>MSPILAKNIVYVAQIKGQITSYTYDQFDRYITIAEQDNAEAIIIELDTPGGRADAMMNIVQRIQQSKIPVIIYVYPPGASAASAGTYIALGSHLIAMAPGTSIGACRPILGYSQNGSIIEAPPKITN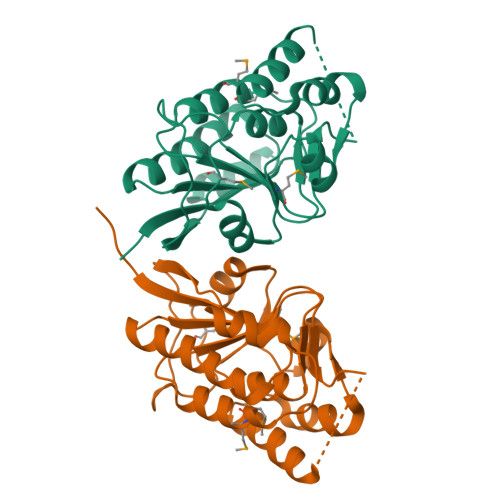YFIAYIKSLAQESGRNATIAEEFITKDLSLTPEEALKYGVIEVVARDINELLKKSNGMKTKIPVNGRYVTLNFTNVEVRYLAPSFKDKLISYITDLEHHHHHH[2x]>MGSSHHHHHHGSSLEVLFQGPGSLAKRIIASLDVKDGRVVKGSNFENLRDSGDPVELGKFYSEIGIDELVFLDITASVEKRKTMLELVEKVAEQIDIPFT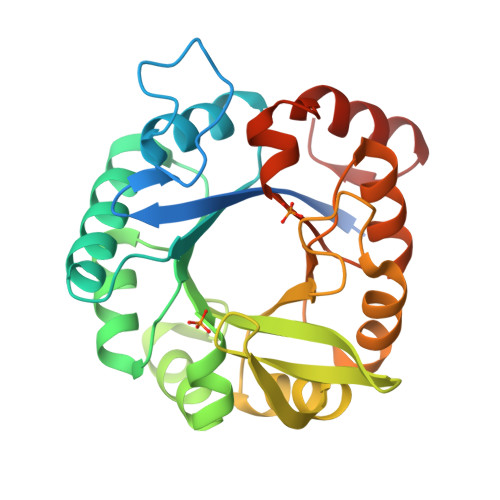VGGGIHDFETASELILRGADKVSINTAAVENPSLITQIAQTFGSQAVVVAIDAKRVDGEFMVFTYSGKKNTGILLRDWVVEVEKRGAGEILLTSIDRDGTKSGYDTEMIRFVRPLTTLPIIASGGAGKMEHFLEAFLAGADAALAASVFHFREIDVRELKEYLKKHGVNVRLEGL[2x]> GPDSMSIDIHSFIATHPLNLTCLFLGDTNAGKSTLLGHLLYDLNEISMSSMRELQKKSSNLDPSSSNSFKVILDNTKTERENGFSMFKKVIQVENDLLPPSSTLTLIDTPGSIKYFNKETLNSILTFDPEVYVLVIDCNYDSWEKSLDGPNNQIYEILKVISYLNKNSACKKHLIILLNKADLISWDKHRLEMIQSE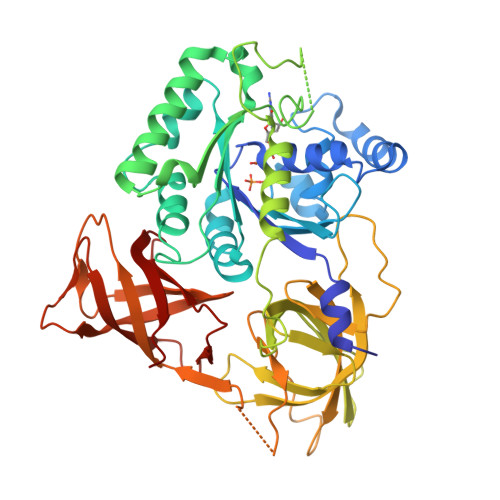LNYVLKENFQWTDAEFQFIPCSGLLGSNLNKTENITKSKYKSEFDSINYVPEWYEGPTFFSQLYLLVEHNMNKIETTLEEPFVGTILQSSVLQPIAEINYVSLKVLINSGYIQSGQTIEIHTQYEDFHYYGIVSRMKNSKQILETNTKNNISVGLNPDILEVLVKIHNTEDFTKKQFHIRKGDIIIHSRKTNTLSPNLPNTLKLLALRLIKLSIQTHALSDPVDLGSELLLYHNLTHNAVKLVKILGTNDISINPNQSLIVEVEIIEPDFALNVIDSKYITNNIVLTSIDHKVIAVGRIACQ>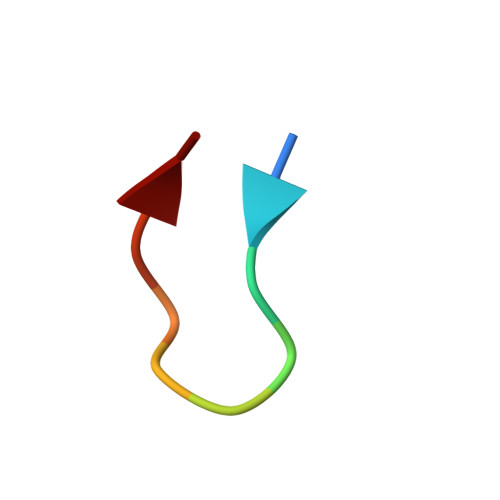 YYDPETGTWY>SRAYDLVVIGAGSGGLEAGWNAASLHKKRVAVIDLQKHHGPPHYAALGGTCVNVGCVPKKLMVTGANYMDTIRESAGFGWELDRESVRPNWKALIAAKNKAVSGINDSYEGMFADTEGLTFHQGFGALQDNHTVLVRESADPNSAVLETLDTEYILLATGSWPQHLGIEGDDLCITSNEAFYLDEAPKRALCVGGGYISIEFAGIFNAYKARGGQVDLAYRGDMILRGFDSELRKQLTEQLRANGINVRTHENPAKVTKNADGTRHVVFESGAEADYDVVMLAIGRVPRSQTLQLEKAGVEVAKNGAIKV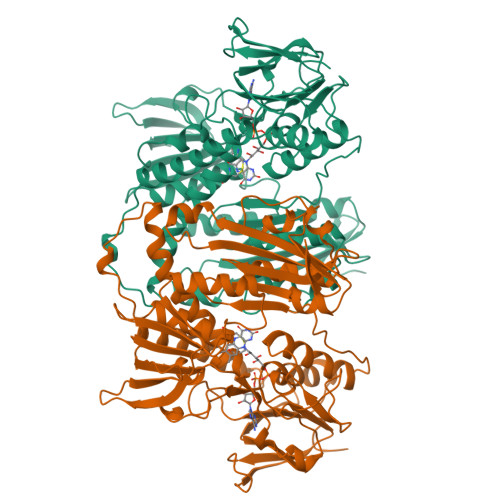DAYSKTNVDNIYAIGDVTDRVMLTPVAINEGAAFVDTVFANKPRATDHTKVACAVFSIPPMGVCGYVEEDAAKKYDQVAVYESSFTPLMHNISGSTYKKFMVRIVTNHADGEVLGVHMLGDSSPEIIQSVAICLKMGAKISDFYNTIGVHPTSAEELCSMRTPAYFYEKGKRVEKIDSNL[4x]>GSHMGIQETDPLTQLSLPPGFRFYPTDEELMVQYLCRKAAGYDFSLQLIAEIDLYKFDPWVLPNKALFGEKEWYFFSPRDRKYPNGSRPNRVAGSGYWKATGTDKIISTEGQRVGIKKALVFYIGKAPKGTKTNWIMHEYRLIEPSRRNGSTKLDDWVLCRIYKKQSSAQK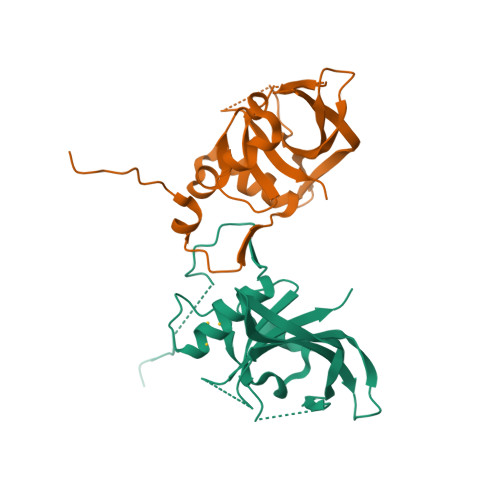[2x]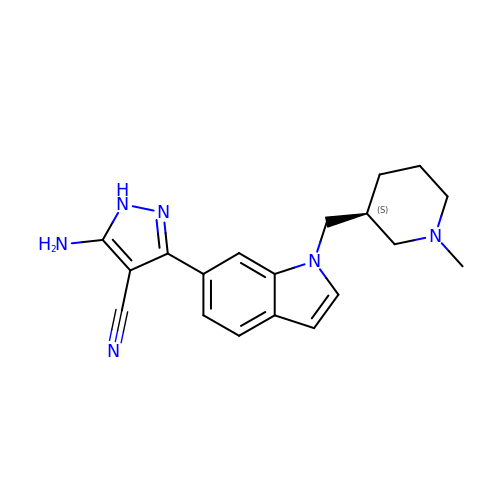5-azanyl-3-[1-[[(3~{S})-1-methylpiperidin-3-yl]methyl]indol-6-yl]-1~{H}-pyrazole-4-carbonitrile | C19 H22 N6 | AJRDTQMINSKQOE-ZDUSSCGKSA-N> KELLDADGDILRNGGTYYIVPAFRGKGGGLTLAKIGDESCPLNVVQAESETKRGLPAMIWTPPRIAILTPAFYLNIEFQPRDPPACLQKYGRLSWKVEGE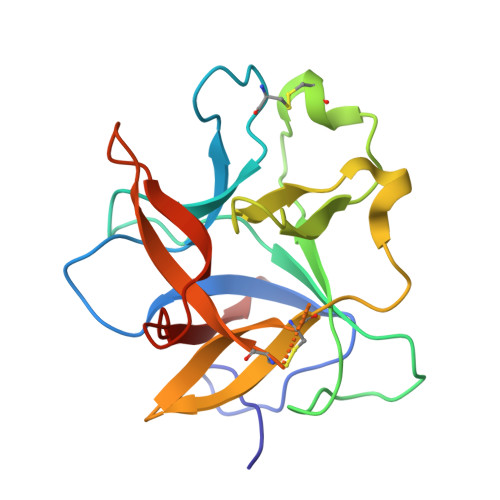SQEVKIAPASEQHLFGSFKIEPYRDDYKLVYCEGNSDDESCKDLGISIDDENNRLLVVKDGDPLAVRFEKSK C-terminal Src kinase (Csk) and Csk-homologous kinase (Chk) are members of the CSK family of protein tyrosine kinases. These proteins suppress the activity of Src family kinases (SFKs) by selectively phosphorylating the conserved C-terminal tail regulatory tyrosine. Csk and Chk both contain SH3, SH2, and kinase domains, which are separated by the SH3–SH2 and SH2-kinase linkers. The Csk SH2 domain is crucial in stabilizing the kinase domain in the active conformation.

Mills et al. studied the unique disulfide bond of Csk SH2 that is absent in other known SH2 domains. Crystal structures of both oxidized SH2 and C122S SH2 were solved and refined. As the structure refinement for the oxidized form of L-SH2 progressed, the maps indicated dual conformations for the residue C122, which were successfully modeled as such. Therefore, the high-resolution structures of oxidized L-SH2 reveal dual conformations of disulfide bond that were not observed in the lower-resolution structure of full-length Csk. X-ray crystallography data were also consistent with the NMR observation, in which most of the changes in chemical shift took place in the residues close to C122, and this area was likely to undergo greater structural change than in the C164 residue area. The S–S distance of the disulfide bond was 2.0 Å, whereas the O–S distance in the C122S mutant was 3.7 Å. Formation of the disulfide bond assisted in the packing of αB to the hydrophobic region of the protein consisting of βC and βD. The disulfide bond formation significantly enhances the thermal stability of SH2 domain and assists in the packing of αB into the hydrophobic region of the protein consisting of βC and βD. The crystal structure also revealed that the linker region fold back on the SH2 domain. Additionally, the hydrophobic interactions between L77 in the linker and L149, F83, and Y116 make the linker fold back to the SH2 and thus stabilizing the structure.

> AGTKLSLMPWFHGKITREQAERLLYPPETGLFLVRESTNYPGDYTLCVSCDGKVEHYRIMYHASKLSIDEEVYFENLMQLVEHYTSDADGLCTRLIKPKVMEGTVA> MALRGTV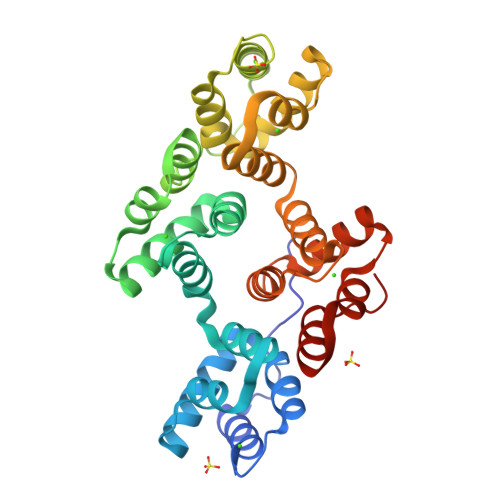TDFSGFDGRADAEVLRKAMEGLGTDEDSILNLLTARSNAQRQQIAEEFKTLFGRDLVNDMKSELTGKFEKLIVALMKPSRLYDAYELKHALKGAGTDEKVLTEIIASRTPEELRAIKQAYEEEYGSNLEDDVVGDTSGYYQRMLVVLLQANRDPDTAIDDAQVELDAQALFQAGELKWGTDEEKFITILGTRSVSHLRRVFDKYMTISGFQIEETIDRETSGNLENLLLAVVKSIRSIPAYLAETLYYAMKGAGTDDHTLIRVIVSRSEIDLFNIRKEFRKNFATSLYSMIKGDTSGDYKKALLLLCGGEDD>[2x]MGRVEVRVEFEGDKMR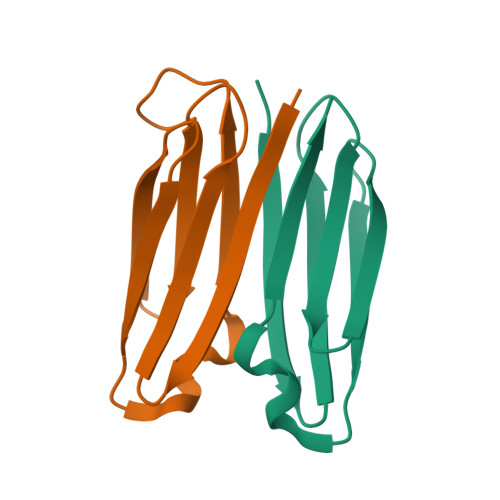VRLRNDSSTPVEVHIKVGDEKRTVTVNPGEEVEVTFSANDPHKFNRPQFTIEWGGQRQHFQHHHHHH>[6x]GDTEKKV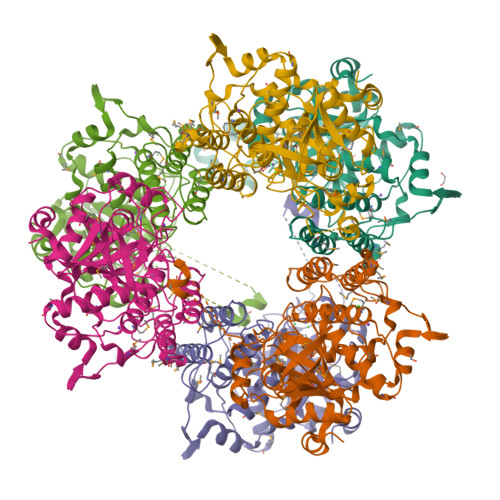SEEGFVFTTVKENPITSVKNQNRAGTCWCYSSYSFLESELLRMGKGEYDLSEMFTVYNTYLDRADAAVRTHGDVSFSQGGSFYDALYGMETFGLVPEEEMRPGMMYADTLSNHTELSALTDAMVAAIAKGKLRKLQSDENNAMLWKKAVAAVHQIYLGVPPEKFTYKGKEYTPKSFFESTGLKASDYVSLTSYTHHPFYTQFPLEIQDNWRHGMSYNLPLDEFMEVFDNAINTGYTIAWGSDVSESGFTRDGVAVMPDDEKVQELSGSDMAHWLKLKPEEKKLNTKPQPQKWCTQAERQLAYDNYETTDDHGMQIYGIAKDQEGNEYYMVKNSWGTNSKYNGIWYASKAFVRYKTMNIVVHKDALPKAIKAKLGIK Pendrin (SLC26A4) is an anion exchanger expressed in the apical membranes of selected epithelia. Encoded by the gene SLC26A4, pendrin belongs to the solute carrier 26 (SLC26) family. Pendrin ablation causes Pendred syndrome, a genetic disorder associated with sensorineural hearing loss, hypothyroid goiter, and reduced blood pressure.

Similarly, the pendrin sample in the anion pair of Cl−/I− (1:3) (pendrin-Cl/I) was prepared and used for structure determination. Symmetric inward-open and asymmetric homodimers were observed with approximate percentage of 75 and 25%, respectively. After superimposing all structures we resolved, we found very little difference among inward-open structures or among outward-open structures, respectively, with root mean squared deviation (RMSD) no more than 0.5 Å. The asymmetric homodimer consists of one inward-facing protomer and the other outward-facing protomer, representing coincident uptake and secretion- a unique state of pendrin as an electroneutral exchanger. Considering the significant cross-section area increase from inward-open state to outward-open state, we hypothesize that when one protomer is outward-open, the other one would be inward-open to minimize their effects on the outer leaflet. Therefore, the coincidence of secretion and uptake in this asymmetric homodimer shapes the molecular basis of the electroneutral exchange of pendrin with an inverted alternate-access mechanism.

>[2x]MAARGGRSEPPQLAEYSCSYTVSRPVYSELAFQQQRERRLPERRTLRDSLARSCSCSRKRAFGVVKTLLPILDWLPKYRVKEWLLSDIISGVSTGLVGTLQGMAYALLAAVPVQFGLYSAFFPILTYFVFGTSRHISVGPFPVVSLMVGSVVLSMAPDDHFLVPSGNGSALNSTTLDTGTRDAARVLLASTLTLLVGIIQLVFGGLQIGFIVRYLADPLVGGFTTAAAFQVLVSQLKIVLNVSTKNYNGILSIIYTLIEIFQNIGDTNIADFIAGLLTIIVCMAVKELNDRFKHRIPVPIPIEVIVTIIATAISYGANLEKNYNAGIVKSIPSGFLPPVLPSVGLFSDMLAASFSIAVVAYAIAVSVGKVYATKHDYVIDGNQEFIAFGISNVFSGFFSCFVATTALSRTAVQESTGGKTQVAGLISAVIVMVAIVALGRLLEPLQKSVLAAVVIANLKGMFMQVCDVPRLWKQNKTDAVIWVFTCIMSIILGLDLGLLAGLLFALLTVVLRVQFPSWNGLGSVPSTDIYKSITHYKNLEEPEGVKILRFSSPIFYGNVDGFKKCINSTVGFDAIRVYNKRLKALRRIQKLIKKGQLRATKNGIISDIGSSNNAFEPDEDVEEPEELNIPTKEIEIQVDWNSELPVKVNVPKVPIHSLVLDCGAVSFLDVVGVRSLRMIVKEFQRIDVNVYFALLQDDVLEKMEQCGFFDDNIRKDRFFLTVHDAILHLQNQVKSREGQDSLLETVARIRDCKDPLDLMEAEMNAEELDVQDEAMRRLAS> MAAPLGGMFSGQPPGPPQAPPGLPGQASLLQAAPGAPRPSSSTLVDELESSFEACFASLVSQDYVNGTDQEEIRTGVDQCIQKFLDIARQTECFFLQKRLQLSVQKPEQVIKEDVSELRNELQRKD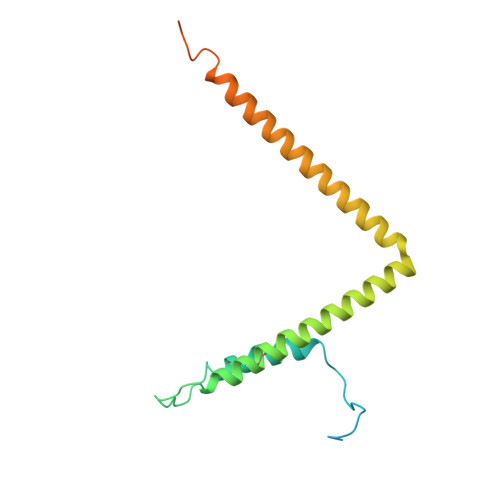ALVQKHLTKLRHWQQVLEDINVQHKKPADIPQGSLAYLEQASANIPAPLKPT methyl 4-sulfamoylbenzoate | C8 H9 N O4 S | 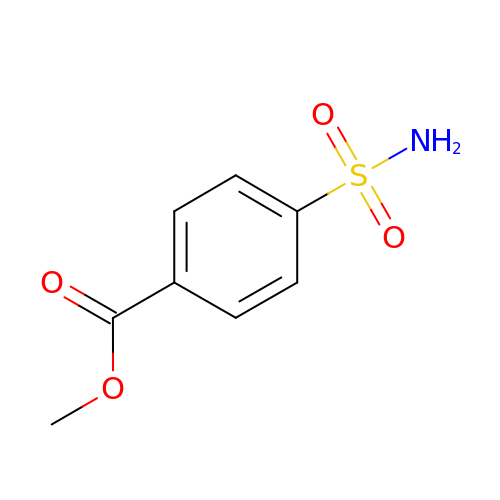XLOVNJUCAFIANM-UHFFFAOYSA-N> GDHYDDELFSDVQDIKTALAKIHEDNQKIISKLESIPKIKGEVESIKKQINRQNISISTLEGHLSSIMIAIP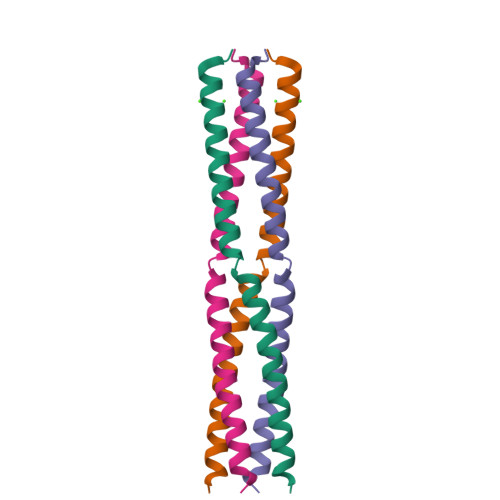HHHHHH>[6x]MGSSHHHHHHSMQGHPEVIDYLNTLLTGELAARDQYFIHSRIYEDWGFSKLYERLNHEMEEET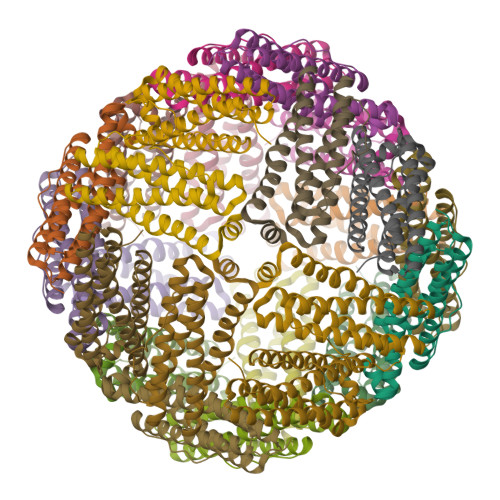QHADALLRRILLLEGTPRMRPDDIHPGTTVPEMLEADLKLERHVRAALAKGIALCEQHKDFVSRDILLAQLRDTEEDHAYWLEQQLGLIARIGLENYLQSQM> MNRIKVAILFGGCSEEHDVSVKSAIEIAANINKEKYEPLYIGITKSGVWKMCE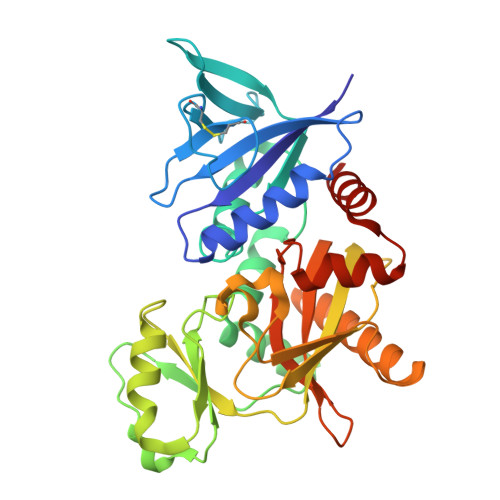KPCAEWENENCYSAVLSPDKKMHGLLVKKNHEYEINHVDVAFSALHGKSGEDGSIQGLFELSGIPFVGCDIQSSAICMDKSLTYIVAKNAGIATPAFWVINKDDRPVAATFTYPVFVKPARSGSSFGVKKVNSADELDYAIESARQYDSKILIEQAVSGCEVGCAVLGNSAALVVGEVDQIRLQYGIFRIHQEVEPEKGSENAVITVPADLSAEERGRIQETVKKIYKTLGCRGLARVDMFLQDRGRIVLNEVNTLPGFTSYSRYPRMMAAAGISLPELIDRLIVLALKG>[2x]MFSAGHKIKGTVVLMPKNELEVNPDGSAVDNLNAFLGRSVSLQLISATKADAHGKGKVGKDTFLEGINTSLPTLGAGESAFNIHFEWDGSMGIPGAFYIKNYMQVEFFLKSLTLEAISNQGTIRFVCNSWVYNTKLYKSVRIFFANHTYVPSETPAPLVEYREEELKSLRGNGTGERKEY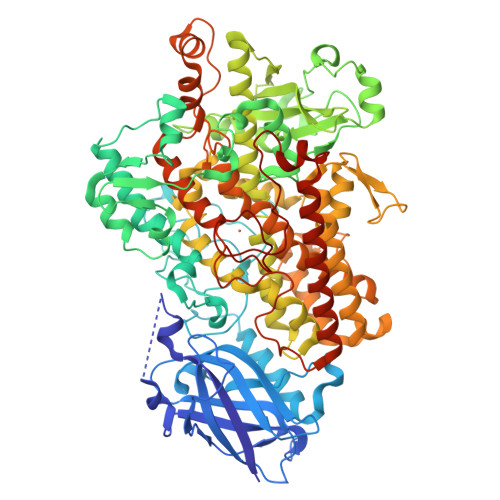DRIYDYDVYNDLGNPDKSEKLARPVLGGSSTFPYPRRGRTGRGPTVTDPNTEKQGEVFYVPRDENLGHLKSKDALEIGTKSLSQIVQPAFESAFDLKSTPIEFHSFQDVHDLYEGGIKLPRDVISTIIPLPVIKELYRTDGQHILKFPQPHVVQVSQSAWMTDEEFAREMIAGVNPCVIRGLEEFPPKSNLDPAIYGDQSSKITADSLDLDGYTMDEALGSRRLFMLDYHDIFMPYVRQINQLNSAKTYATRTILFLREDGTLKPVAIELSLPHSAGDLSAAVSQVVLPAKEGVESTIWLLAKAYVIVNDSCYHQLMSHWLNTHAAMEPFVIATHRHLSVLHPIYKLLTPHYRNNMNINALARQSAINANGIIETTFLPSKYSVEMSSAVYKNWVFTDQALPADLIKRGVAIKDPSTPHGVRLLIEDYPYAADGLEIWAAIKTWVQEYVPLYYARDDDVKNDSELQHWWKEAVEKGHGDLKDKPWWPKLQTLEDLVEVCLIIIWIASALHAAVNFGQYPYGGLIMNRPTASRRLLPEKGTPEYEEMINNHEKAYLRTITSKLPTLISLSVIEILSTHASDEVYLGQRDNPHWTSDSKALQAFQKFGNKLKEIEEKLVRRNNDPSLQGNRLGPVQLPYTLLYPSSEEGLTFRGIPNSISI> MAGQTTVDSRRQPPEEVDVLVVGAGFSGLYALYRLRELGRSVHVIETAGDVGGVWYWNRYPGARCDIESIEYCYSFSEEVLQEWNWTERYASQPEILRYINFVADKFDLRSGITFHTTVTAAAFDEATNTWTVDTNHGDRIRARYLIMASGQLSVPQLPNFPGLKDFAGNLYHTGNWPHEPVDFSGQRVGVIGTGSSGIQVSPQ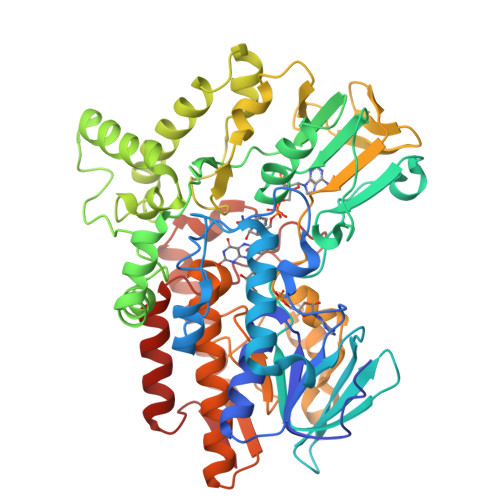IAKQAAELFVFQRTPHFAVPARNAPLDPEFLADLKKRYAEFREESRNTPGGTHRYQGPKSALEVSDEELVETLERYWQEGGPDILAAYRDILRDRDANERVAEFIRNKIRNTVRDPEVAERLVPKGYPFGTKRLILEIDYYEMFNRDNVHLVDTLSAPIETITPRGVRTSEREYELDSLVLATGFDALTGALFKIDIRGVGNVALKEKWAAGPRTYLGLSTAGFPNLFFIAGPGSPSALSNMLVSIEQHVEWVTDHIAYMFKNGLTRSEAVLEKEDEWVEHVNEIADETLYPMTASWYTGANVPGKPRVFMLYVGGFHRYRQICDEVAAKGYEGFVLT>[2x]MSLYEWLNALPKAELHLHLEGTLEPELLFALAERNRIALPWNDVETLRKAYAFNNLQEFLDL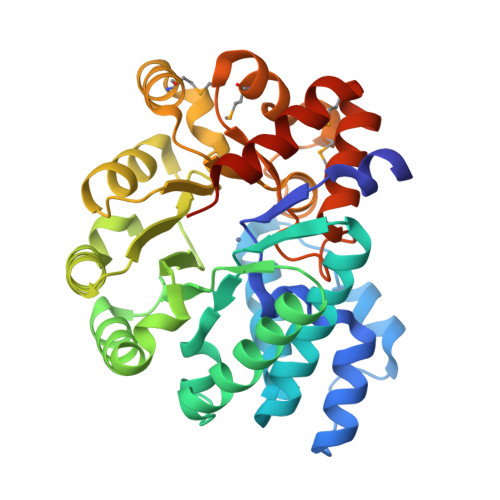YYAGADVLRTEQDFYDLTWAYLQKCKAQNVVHVEPFFDPQTHTDRGIPFEVVLAGIRAALRDGEKLLGIRHGLILSFLRHLSEEQAQKTLDQALPFRDAFIAVGLDSSEVGHPPSKFQRVFDRARSEGFLTVAHAGEEGPPEYIWEALDLLKVERIDHGVRAFEDERLMRRLIDEQIPLTVCPLSNTKLCVFDDMSQHTILDMLERGVKVTVNSDDPAYFGGYVTENFHALQQSLGMTEEQARRLAQNSLDARLVKEGHHHHHH> MEKSLVDTVYALKDEVQELRQDN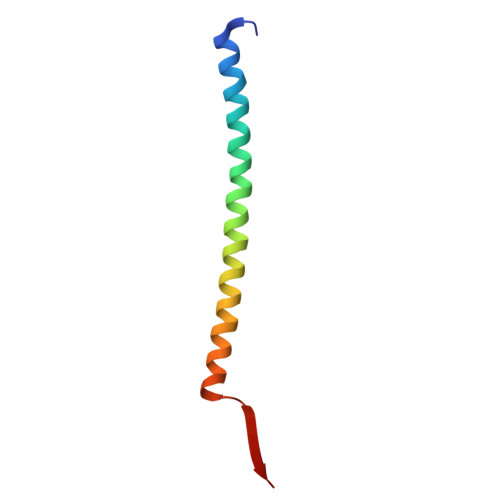KKMKKSLEEEQRARKDLEKLVRKVLKNMNDPAWDETNL>[2x]MAISLATKAATDALKVNRAPVGVEPQEVHKWLQSFNWDFKENRTKYPTKYHMANETKEQFKVIAKEYARMEAAKDERQFGTLLDGLTRLGAGNKVHPRWGETMKVISNFLEVGEYNAIAASAMLWDSATAAEQKNGYLAQVLDEIRHTHQCAFINHYYSKHYHDPAGHNDARRTRAIGPLWKGMKRVFADGFISGDAVECSVNLQLVGEACFTNPLIVAVTEWASANGDEITPTVFLSVETDELRHMANGYQTVVSIANDPASAKFLNTDLNNAFWTQQKYFTPVLGYLFEYGSKFKVEPWVKTWNRWVYEDWGGIWIGRLGKYGVESPASLRDAKRDAYWAHHDLALAAYAMWPLGFARLALPDEEDQAWFEANYPGWADHYGKIFNEWKKLGYEDPKSGFIPYQ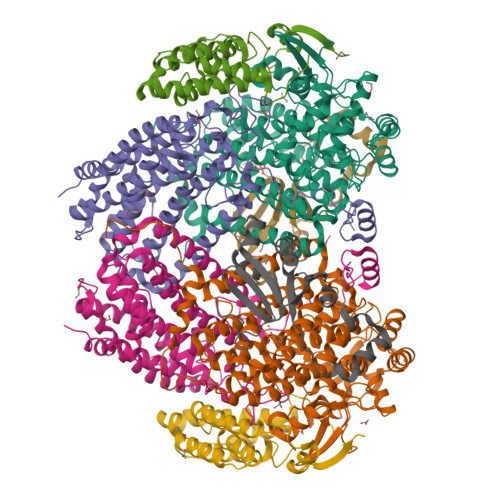WLLANGHDVYIDRVSQVPFIPSLAKGTGSLRVHEFNGKKHSLTDDWGERQWLIEPERYECHNVFEQYEGRELSEVIAEGHGVRSDGKTLIAQPHTRGDNLWTLEDIKRAGCVFPDPLAKF;>[2x]MSQPQSSQVTKRGLTDPERAAIIAAAVPDHALDTQRKYHYFIQPRWKRLSEYEQLSCYAQPNPDWIAGGLDWGDWTQKFHGGRPSWGNESTELRTTDWYRHRDPARRWHHPYVKDKSEEARYTQRFLAAYSSEGSIRTIDPYWRDEILNKYFGALLYSEYGLFNAHSSVGRDCLSDTIRQTAVFAALDKVDNAQMIQMERLFIAKLVPGFDASTDVPKKIWTTDPIYSGARATVQEIWQGVQDWNEILWAGHAVYDATFGQFARREFFQRLATVYGDTLTPFFTAQSQTYFQTTRGAIDDLFVYCLANDSEFGAHNRTFLNAWTEHYLASSVAALKDFVGLYAKVEKVAGATDRAGVSEALQRVFGDWKIDYADKIGFRVDVDQKVDAVLAGYKN;>[2x]MAKREPIHDNSIRTEWEAKIAKLTSVDQATKFIQDFRLAYTSPFRKSYDIDVDYQYIERKIEEKLSVLKTEKLPVADLITKATTGEDAAAVEATWIAKIKAAKSKYEAERIHIEFRQLYKPPVLPVNVFLRTDAALGTVLMEIRNTDYYGTPLEGLRKERGVKVLHLQA;>[2x]MSSAHNAYNAGIMQKTGKAFADEFFAEENQVVHESNAVVLVLMKSDEIDAIIEDIVLKGGKAKNPSIVVEDKAGFWWIKADGAIEIDAAEAGELLGKPFSVYDLLINVSSTVGRAYTLGTKFTITSELMGLDRALTDI> SELDA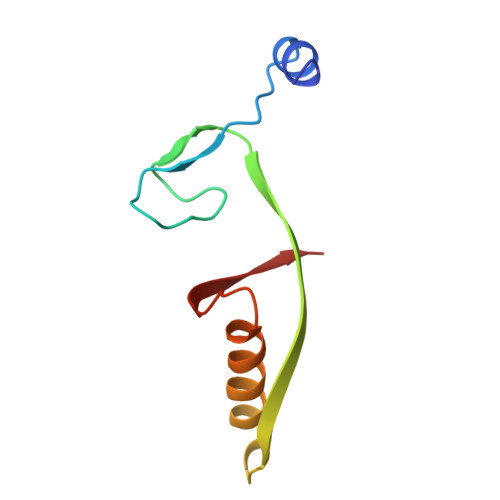KLNKLGVDRIAISPYKQWTRGYMEPGNIGNGYVTGLKVDAGVRDKSDDDVLDGIVSYDRAETKNAYIGQINMTTAS> PENNKFKVKPLPYAYDALEPYIDKETMKLHHDKHYQAYVDKLNA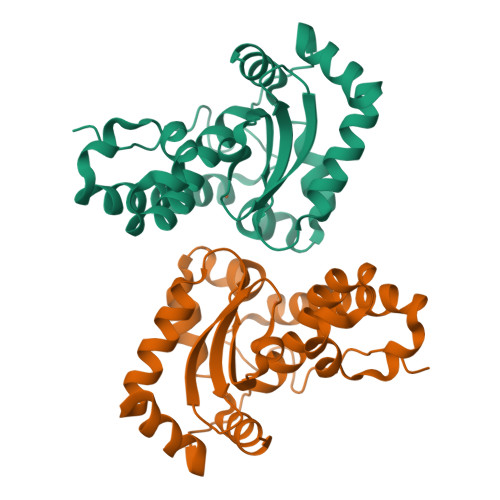ALEKYPELYNYSLCELLQNLDSLPKDIATTVRNNAGGAYNHKFFFDIMTPEKTIPSESLKEAIDRDFGSFEKFKQEFQKSALDVFGSGWAWLVATKDGKLSIMTTPNQDSPVSKNLTPIIGLDVWEHAYYLKYQNRRNEYIDNWFNVVNWNGALENYKNLKSQD> MGVRWTLWDTLAFLLLLSLLLPSLLIMFIPSTFKRPVSSWKARNLRKTLLMASSVRLKPLNCSRLPCVYAQETLTF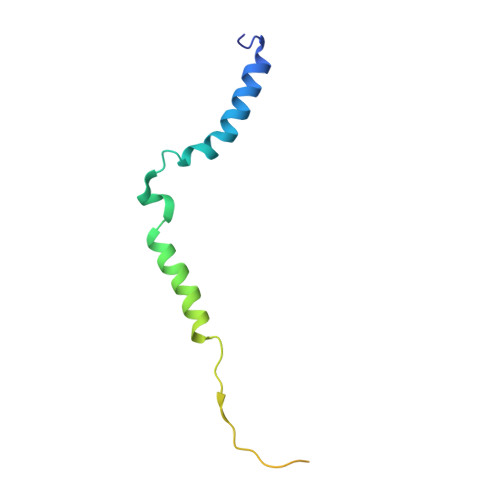LLTQKKTCVKNYVRKEHHHHHH(6R,6aR,7S,10R,10aS)-6-(3,5-bis(trifluoromethyl)phenyl)-5,6,6a,7,8,9,10,10a-octahydro-7,10-methanophenanthridine-3-carboxylic 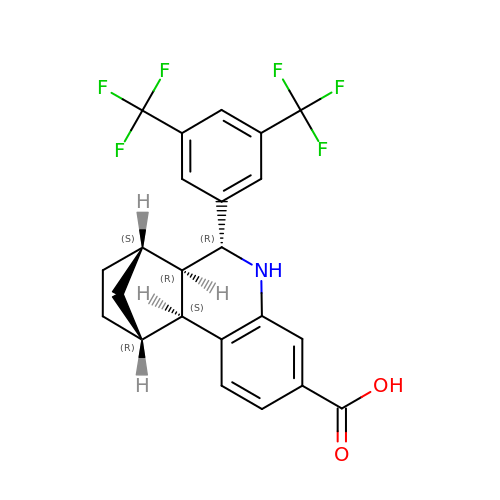acid | C23 H19 F6 N O2 | GGGBDYORXLHJAW-JMDSXHSASA-N methyl 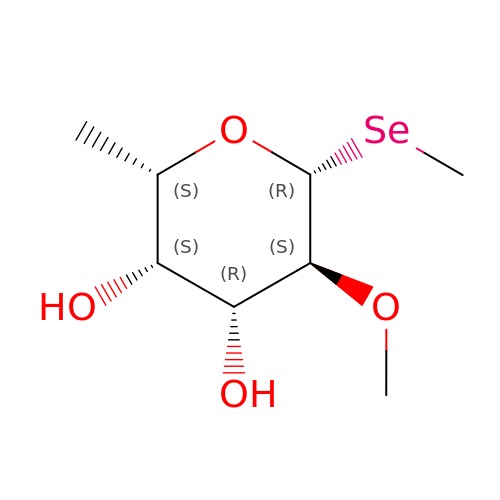1-seleno-2-O-methyl-beta-L-fucopyranoside | C8 H16 O4 Se | JGCHFCAEXBTPJU-FMGWEMOISA-N>MTTHIQKPATGSPLTLLNGVLQVPDQPIIPFIEGDGIGCDVTPAMRSVVDAAVAKVYGGQRQIAWMELFAGQKAVQLYGEGQYLPDETMAAIREYKVAIKGPLETPVGGGIRSLNVAMRQDLDLYVCLRPVRYFEGTPSPMRHPEKVDMVIFRENSEDIYAGIEWPAGSPEAEKIIRFLREEMGVTKIRFPDSSAIGIKPVSTEGSERLIRRTIQYALEHGKPSVSLVHKGNIMKFTEGGFRDWGYALAEREFAGRVFTWRQKAAISKAEGKAAGQKAEQQAIAD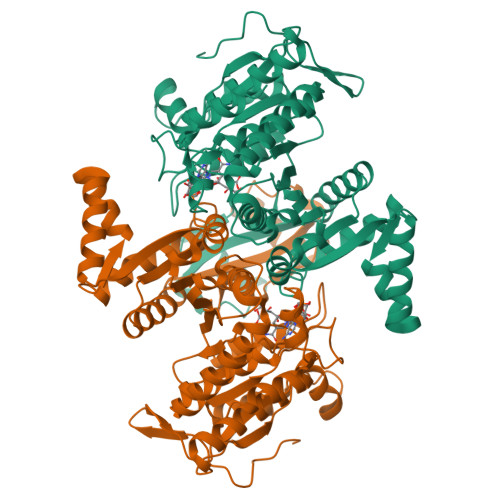GKLIIKDVIADNFLQQILLRPEDYSVVATLNLNGDYVSDALAAEVGGIGMAPGANLSDTHAIFEATHGTAPDIAGQGKANPSSLILSAVMMLEHLGWGEAAQAIVAAMNATIAAGEVTGDLAALRGDVPALSTTEFTAALIRRF[4x]>MTSITPVTLANCEDEPIHVPGAIQPHGALVTLRADGMVLAASENIQALLGFVASPGSYLTQEQVGPEVLRMLEEGLTGNGPWSNSVETRIGEHLFDVIGHSYKEVFYLEFEIRTADTLSITSFTLNAQRIIAQVQLHNDTASLLSNVTDELRRMTGYDRVMAYRFRHDDSGEVVAESRREDLESYLGQRYPASDIPAQARRLYIQNPIRLIADVAYTPMRVFPALNPETNESFDLSYSVLRSVSPIHCEYLTNMGVRASMSISIVVGGKLWGLFSCHHMSPKLIPYPVRMSFQIFSQVCSAIVERLEQGRIAELLRVSTERRLALARRARDADDLFGALAHPDDGIAALIPCDGALVMLGGRTLSIRGDFERQAGNVLQRLQR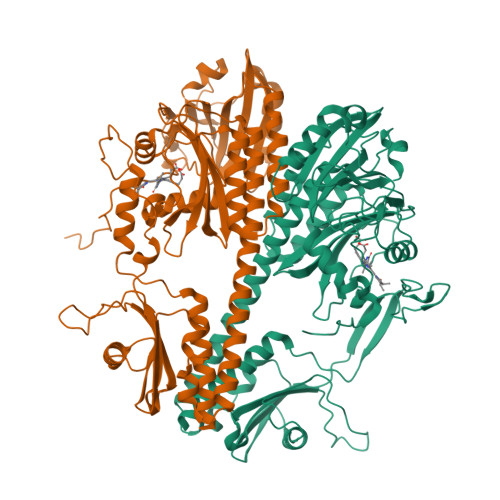DPERDIYHTDNWPQPSEDSPDGGDCCGVLAIRFHRQESGWIFWFRHEEVHRIRWGGKPEKLLTIGPSGPRLTPRGSFEAWEEVVRGHSTPWSETDLAIAEKLRLDLMELCLNHAAEVDRMRQRLIAVLGHDLRNPLQSISMAAALLSSSDTRTTELRQHISASSSRMERLVSQILDMSRLQSGIGLTVNPVDTDVSQLVRQIVCETDVAYPGLVIEIAIDPQVRAVVDPDRYAQVAANLLSNARHHGLPGRPVLVTLTRQGDEVCLSVLNETSGLSEAQLANLFEPFKRESADNQRNRNGLGIGLYISQAIAQAHQGRIDVDCRDDVITFCLRLPVRQAETGSSS[2x]> MCWAAAIPIAISGAQAIS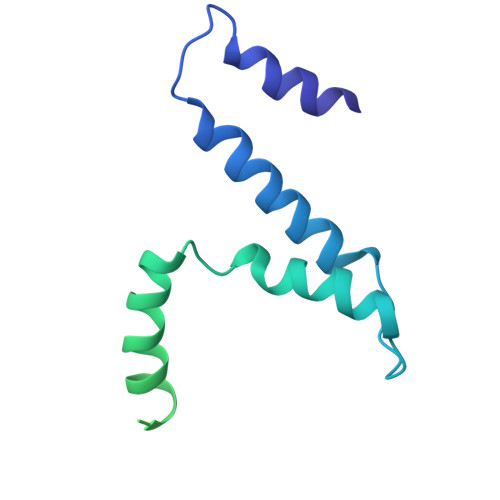GQNAQAKMIAAQTAAGRRQAMEIMRQTNIQNADLSLQARSKLEEASAELTSQNMQKVQAIGSIRAAIGESMLEGSSMDRIKRVTEGQFIREANMVTENYRRDYQAIFAQQLGGTQSAASQIDEIYKSEQKQKSKLQMVLDPLAIMGSSAASAYASGAFDSKSTTKAPIVAAKGTKTGR N,3-DIHYDROXYBENZAMIDE 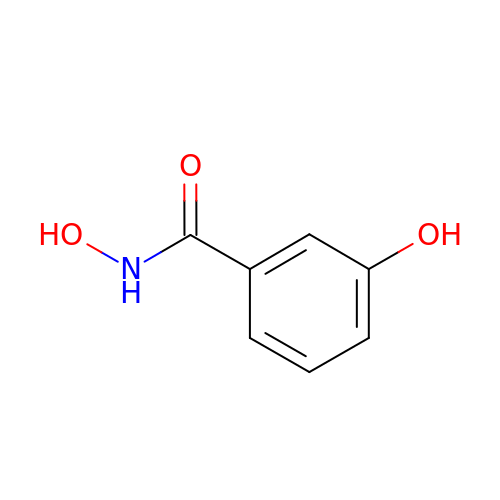| C7 H7 N O3 | IRGXGFPSYHAJER-UHFFFAOYSA-N>[2x]MSFEEFTPLNEKSLVDYIKSTPALSSKIGADKSDDDLVIKEVGDGNLNFVFIVVGSSGSLVIKQALPYIRCIGESWPMTKERAYFEATTLRKHGNLSPDHVPEVYHFDRTMALIGMRYLEPPHIILRKGLIAGIEYPFLADHMSDYMAKTLFFTSLLYHDTTEHRRAVTEFCGNVELCRLTEQVVFSDPYRVSTFNRWTSPYLDDDAKAVREDSALKLEIAELKSMFCERAQALIHGDLHTGSVMVTQDSTQVIDPEFSFYGPMGFDIGAYLGNLILAFFAQDGHATQENDRKEYKQWILRTIEQTWNLFNKRFIALWDQNKDGPGEAYLADIYNNTEVLKFVQENYMRNLLHDSLGFGAAKMIRRIVGVAHVEDFESIEEDKRRAICERSALEFAKMLLKERRKFKSIGEVVSAIQQQS

To promptly remove the toxic by-product MTA and to ensure sufficient supply of methionine and SAM, a methionine salvage pathway that recycles the methylthio moiety of MTA to methionine has evolved in almost all organisms. In this cycle MTA is first depurinated to 5-methylthioribose (MTR), and then phosphorylated to form MTR 1-phosphate (MTR 1-P). In bacteria and plant cells, two enzymes, MTA nucleosidase and MTR kinase, are required to convert MTA to MTR-1-P while in mammalian cells, MTA phosphorylase phosphorylizes MTA to MTR 1-P in a single step. The bilobal structural organization as well as the topology profile of MTR kinase is consistent with that found in eukaryotic protein kinases.

The structure of Arabidopsis thaliana MTR kinase co-crystallized with ATPγS and MTR has been determined at 1.9 Å resolution. The A. thaliana MTR kinase complex was prepared by co-crystallization with excess but equal amount of ATPγS and MTR, but surprisingly, ADP and MTR were found in the active site. The structure of A. thaliana MTR kinase has two subunits in the asymmetric unit related by a non-crystallographic 2-fold. The nucleotide binds in the cleft region between the two lobes of the protein. In the A. thaliana MTR kinase structure, two Mg(II) ions assist in the binding of the ADP. In A. thaliana MTR kinase, MTR is bound in the higher energy α-ribofuranose anomer with the substrate's O1 hydroxyl cis to the O2 and O3 hydroxyl groups. The O1 and O2 oxygens of MTR form hydrogen bonds (~2.7 Å) with the carboxyl oxygens of D238 of the strictly conserved HGD-motif; while the O2 and O3 oxygens of MTR forms heteronuclear hydrogen bonds (~2.9 Å) with the guanidium nitrogens of R365 of the strictly conserved twin arginine RR-motif. The second arginine R366 does not interact directly with MTR but may facilitate the release of the anionic product, MTR 1-P. In the A. thaliana enzyme, a lysine (K362) is located near the RR-motif, and to mitigate the electrostatic repulsion between these three positively charged residues, a chloride ion is found interacting with K362. The G-loop of A. thaliana MTR kinase has an extended conformation, with interactions formed between N46 and the O4 oxygen of MTR. A consequence of this extended G-loop in the Arabidopsis enzyme is that it shields the active site from solvent, a feature that more closely resembles a eukaryotic protein kinase active site than that of the B. subtilis MTR kinase.>[2x]MTSKVYDPEQRKRMITGPQWWARCKQMNVLDSFINYYDSEKHAENAVIFLHGNATSSYLWRHVVPHIEPVARCIIPDLIGMGKSGKSGNGSYR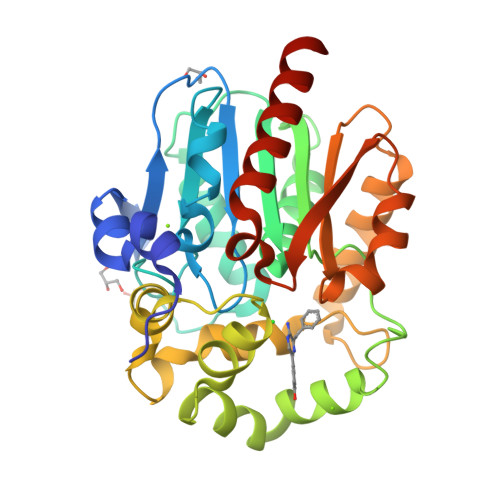LLDHYKYLTAWFELLNLPKKIIFVGHAWGAALAFHYAYEHQDRIKAIVHMESVVDVIESWDEWPDIEEDIALIKSEEGEKMVLENNFFVETVLPSKIMRKLEPEEFAAYLEPFKEKGEVRRPTLSWPREIPLVKGGKPDVVQIVRNYNAYLRASDDLPKLFIESDPGFFSNAIVEGAKKFPNTEFVKVKGLHFLQEDAPDEMGKYIKSFVERVLKNEQHHHHHH>MADYEAKLAKYQADLAKYQKDLAEYPQKLKEYNEEQAKIKEALKKLEQDKNKDGHLTEPSAQSLVYDSEPDAKLSLTTEDGTLLKSSVVDEAFSKSTSKAKYDQKILQLDDLDIRGLEKADSATSTVELYGNIGNKSTWTTNVGNNTEVKWGSVLLKRGQSVTATYTNLQKTYYNGKKVSKIVYKYTVDKDSKFQNPSGNVWLGVFSDPTLGVFASAYTGQVEKDTSIFIKNEFTFYDENDQPINFDNALLSVASLNRENNSIEMAKDYTGKFVRISGSSIDEKDGKIYATKTLNFKKGQGGSRWTMYPNGQEGSGWDSSDAPNSWYGAGAVKISGQHNSITLGAISATLVVPSDSVMAVETGKKPNIWY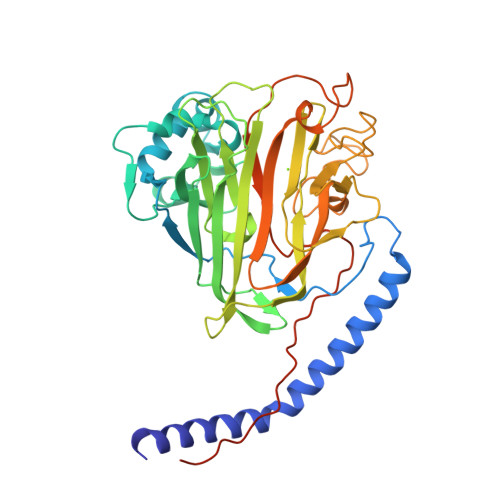SLNGKIRAVNVPKITKENPTPPVEPTAPQAPTENLYFQGLEHHHHHH[2x]> MDAYSTRPLTLSHGSLEHVLLVPTASFFIASQLQEQFNKILPEPTEGFAADDEPTTPAELVGKFLGYVSSLVEPSKVGQFDQVLNLCLTEFENCYLEGNDIHALAAKLLQENDTTLVKTKELIKNYITARIMAKRPFDKKSNSALFRAVGEGNAQLVAIFGGQGNTDDYFEELRDLYQTYHVLVGDLIKFSAETLSELIRTTLDAEKVFTQGLNILEWLENPSNTPDKDYLLSIPISCPLIGVIQLAHYVVTAKLLGFTPGELRSYLKGATGHSQGLVTAVAIAETDSWESFFVSVRKAITVLFFIGVRCYEAYPNTSLPPSILEDSLENNEGVPSPMLSISNLTQEQVQDYVNKTNSHLPAGKQVEISLVNGAKNLVVSGPPQSLYGLNLTLRKAKAPSGLDQSRIPFSERKLKFSNRFLPVASPFHSHLLVPASDLINKDLVKNNVSFNAKDIQIPVYDTFDGSDLRVLSGSISERIVDCIIRLPVKWETTTQFKATHILDFGPGGASGLGVLTHRNKDGTGVRVIVAGTLDINPDDDYGFKQEIFDVTSNGLKKNPNWLEEYHPKLIKNKSGKIFVETKFSKLIGRPPLLVPGMTPCTVSPDFVAATTNAGYTIELAGGGYFSAAGMTAAIDSVVSQIEKGSTFGINLIYVNPFMLQWGIPLIKELRSKGYPIQFLTIGAGVPSLEVASEYIETLGLKYLGLKPGSIDAISQVINIAKAHPNFPIALQWTGGRGGGHHSFEDAHTPMLQMYSKIRRHPNIMLIFGSGFGSADDTYPYLTGEWSTKFDYPPMPFDGFLFGSRVMIAKEVKTSPDAKKCIAACTGVPDDKWEQTYKKPTGGIVTVRSEMGEPIHKIATRGVMLWKEFDETIFNLPKNKLVPTLEAKRDYIISRLNADFQKPWFATVNGQARDLATMTYEEVAKRLVELMFIRSTNSWFDVTWRTFTGDFLRRVEERFTKSKTLSLIQSYSLLDKPDEAIEKVFNAYPAAREQFLNAQDIDHFLSMCQNPMQKPVPFVPVLDRRFEIFFKKDSLWQSEHLEAVVDQDVQRTCILHGPVAAQFTKVIDEPIKSIMDGIHDGHIKKLLHQYYGDDESKIPAVEYFGGESPVDVQSQVDSSSVSEDSAVFKATSSTDEESWFKALAGSEINWRHASFLCSFITQDKMFVSNPIRKVFKPSQGMVVEISNGNTSSKTVVTLSEPVQGELKPTVILKLLKENIIQMEMIENRTMDGKPVSLPLLYNFNPDNGFAPISEVMEDRNQRIKEMYWKLWIDEPFNLDFDPRDVIKGKDFEITAKEVYDFTHAVGNNCEDFVSRPDRTMLAPMDFAIVVGWRAIIKAIFPNTVDGDLLKLVHLSNGYKMIPGAKPLQVGDVVSTTAVIESVVNQPTGKIVDVVGTLSRNGKPVMEVTSSFFYRGNYTDFENTFQKTVEPVYQMHIKTSKDIAVLRSKEWFQLDDEDFDLLNKTLTFETETEVTFKNANIF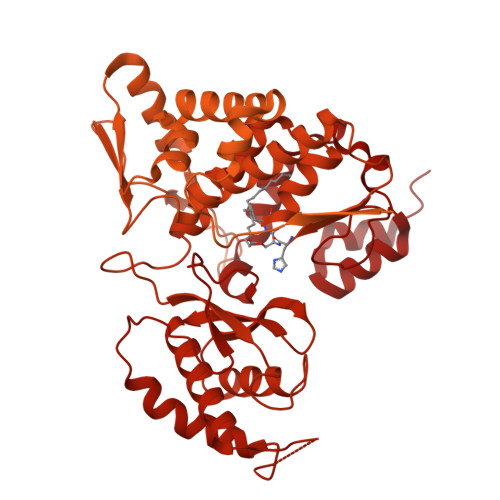SSVKCFGPIKVELPTKETVEIGIVDYEAGASHGNPVVDFLKRNGSTLEQKVNLENPIPIAVLDSYTPSTNEPYARVSGDLNPIHVSRHFASYANLPGTITHGMFSSASVRALIENWAADSVSSRVRGYTCQFVDMVLPNTALKTSIQHVGMINGRKLIKFETRNEDDVVVLTGEAEIEQPVTTFVFTGQGSQEQGMGMDLYKTSKAAQDVWNRADNHFKDTYGFSILDIVINNPVNLTIHFGGEKGKRIRENYSAMIFETIVDGKLKTEKIFKEINEHSTSYTFRSEKGLLSATQFTQPALTLMEKAAFEDLKSKGLIPADATFAGHXLGEYAALASLADVMSIESLVEVVFYRGMTMQVAVPRDELGRSNYGMIAINPGRVAASFSQEALQYVVERVGKRTGWLVEIVNYNVENQQYVAAGDLRALDTVTNVLNFIKLQKIDIIELQKSLSLEEVEGHLFEIIDEASKKSAVKPRPLKLERGFACIPLVGISVPFHSTYLMNGVKPFKSFLKKNIIKENVKVARLAGKYIPNLTAKPFQVTKEYFQDVYDLTGSEPIKEIIDNWEKYEQS> TELTLKPGTLTLAQLRAIHAAPVRLQLDASAAPAIDASVACVEQIIAEDRTAYGINTGFGLLASTRIASHDLENLQRSLVLSHAAGIGAPLDDDLVRLIMVLKINSLSRGFSGIRRKVIDALIALVNAEVYPHIPLKGSVGASGDLAPLAHMSLVLLGEGKARYKGQWLSATEALAVAGLEPLTLAAKEGLALLNGTQASTAYALRGLFYAEDLYAAAIACGGLSVEAVLGSRSPFDARIHEARGQRGQIDTAACFRDLLGDSSEVSLSHKNADKVQDPFSLRCQPQVMGACLTQLRQAAEVLGIEANA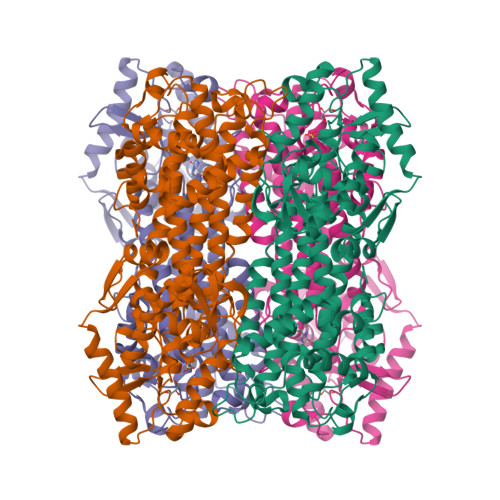VSDNPLVFAAEGDVISGGNFHAEPVAMAADNLALAIAEIGSLSERRISLMMDKHMSQLPPFLVENGGVNSGFMIAQVTAAALASENKALSHPHSVDSLPTSANQEDHVSMAPAAGKRLWEMAENTRGVLAIEWLGACQGLDLRKGLKTSAKLEKARQALRSEVAHYDRDRFFAPDIEKAVELLAKGSLTGLLPAGVLPSL>VETIELKRGSNSVYVQYDDIMFFESSTKSHRLIAHLDNRQIEFYGNLKELSQLDDRFFRCHNSFVVNRHNIESIDSKERIVYF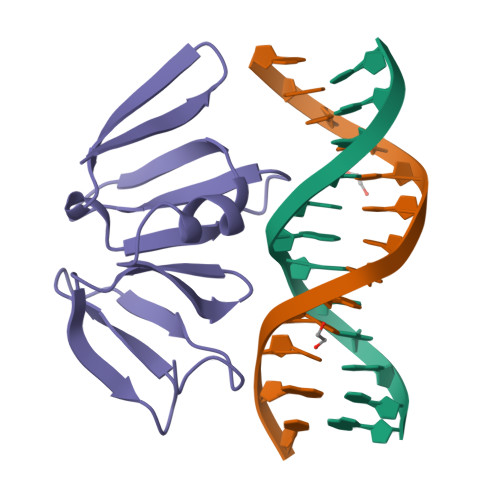KNKEHCYASVRNVKKI[4x]N-{2-[6-(2,4-DIAMINO-6-ETHYLPYRIMIDIN-5-YL)-2,2-DIMETHYL-3-OXO-2,3-DIHYDRO-4H-1,4-BENZOXAZIN-4-YL]ETHYL}ACETAMIDE 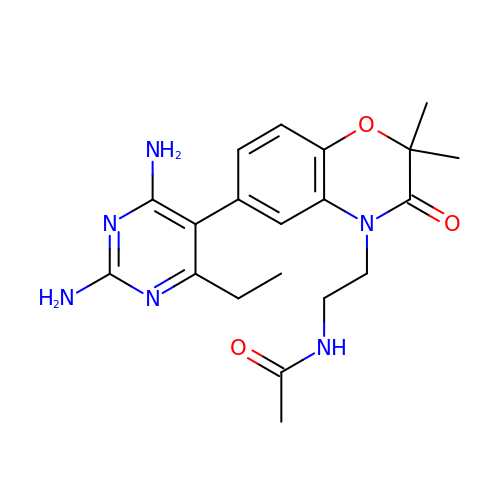| C20 H26 N6 O3 | GBXSOZDYCSBLQX-UHFFFAOYSA-N> METKPRTPVLWLHGLECTCCSESFIRSAHPLAKDVVLSMISLDYDDTLMAAAGHQAEAILEEIMTKYKGNYILAVEGNPPLNQDGMSCIIGGRPFIEQLKYVAKDAKAIISWGSCASWGCVQAAK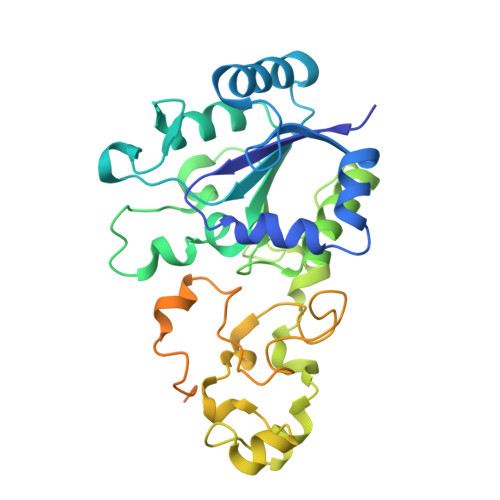PNPTQATPVHKVITDKPIIKVPGCPPIAEVMTGVITYMLTFDRIPELDRQGRPKMFYSQRIHDKCYRRPHFDAGQFVEEWDDESARKGFCLYKMGCKGPTTYNACSTTRWNEGTSFPIQSGHGCIGCSEDGFWDKGSFYDRLTGISQFGVEANADKIGGTASVVVGAAVTAHAAASAIKRASKKNETSGSEHRSAWSHPQFEKRSAWSHPQFEK>MTSAEMTSPNNNSEHQAIAKMRTMIEGFDDISHGGLPIGRSTLVSGTSGTGKTLFSIQFLYNGIIEFDEPGVFVTFEETPQDIIKNARSFGWDLAKLVDEGKLFILDASPDPEGQEVVGGFDLSALIERINYAIQKYRARRVSIDSVTSVFQQYDASSVVRRELFRLVARLKQIGATTVMTTERIEEYGPIARYGVE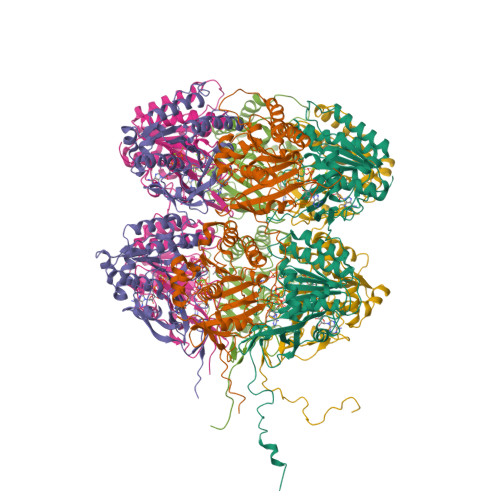EFVSDNVVILRNVLEGERRRRTLEILKLRGTSHMKGEYPFTITDHGINIFPLGAMRLTQRSSNVRVSSGVVRLDEMCGGGFFKDSIILATGATGTGKTLLVSRFVENACANKERAILFAYEESRAQLLRNAYSWGMDFEEMERQNLLKIVCAYPESAGLEDHLQIIKSEINDFKPARIAIDSLSALARGVSNNAFRQFVIGVTGYAKQEEITGLFTNTSDQFMGAHSINDSHISTITDTIILLQYVEIRGEMSRAINVFKMRGSWHDKAIREFMISDKGPDIKDSFRNFERIISGSPTRITVDEKSELSRIVRGVQEKGPES[6x]> MENIQININH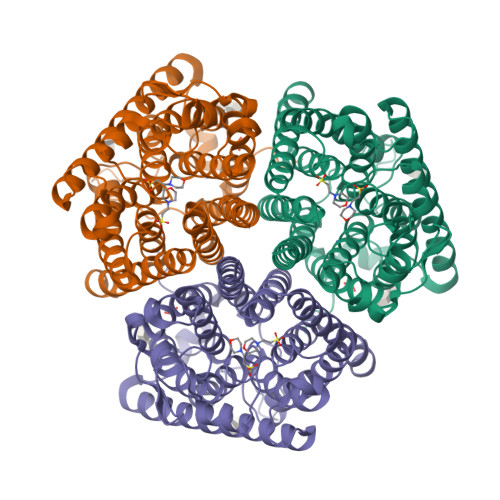LWVIMAACMVFLMQLGFTSYETGFSQSKNAISIALRNLVDTLISSLVFFSVGFGFMFGKSYMGLIGIDLFFANDLALHPNTLSYSFFFFQMVFASTAATILTGAIAERSGFIPNIAGTAFIVAIIYPIFGHWAWGNLFSPDQTGWLKELGFIDFAGATVVHSIGGWFAMAAAIMVGPRIDKYNPDGSSNRIGLHNVPLATLGTFFLWFGWFGFNGGSLLRVSVNIGLVILNTNMAAASAGVSALIFIYATRKRIEAGSLFTAILAGLVAITASSNMVTPVSAVAIGLITGILAIIAEGFIEKTLKIDDPVSAIAVHGVGGVIGTLCVAIFAQKSYLLAENGSRMHQLGIQALGVIVAFSWSFGLGMLFFLCLKKVKRLRVTPEEEKRGLNVAEAA>MPMISCDMRYGRTDE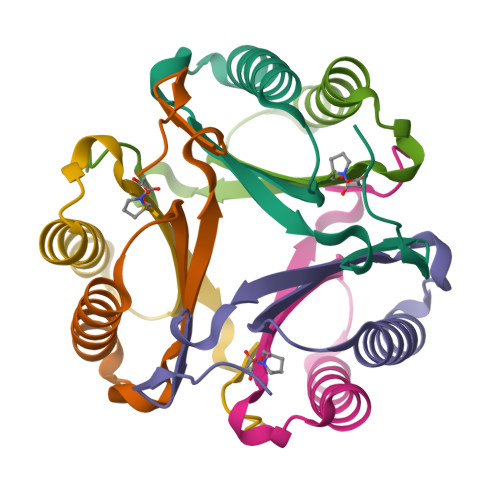QKRALSAGLLRVISEATGEPRENIFFVIREGSGINFVEHGEHLPDYVPGNANDKALIAKLK[6x];>MPFIECHIATGLSVARKQQLIRDVIDVTNKSIGSDPKIINVLLVEHAEANMSISGRIHGEAASTERTPAVS[6x]> KRRRQHGQL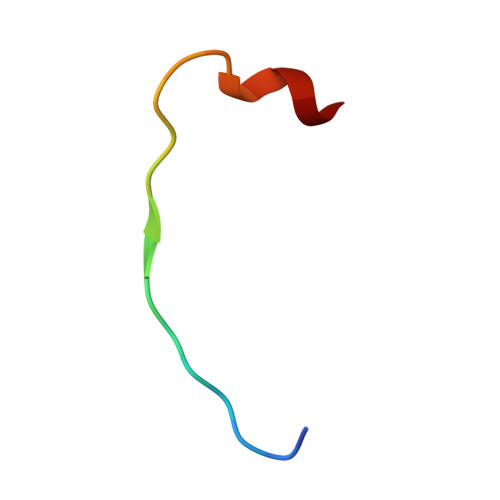WFPEGFKVSE> PAP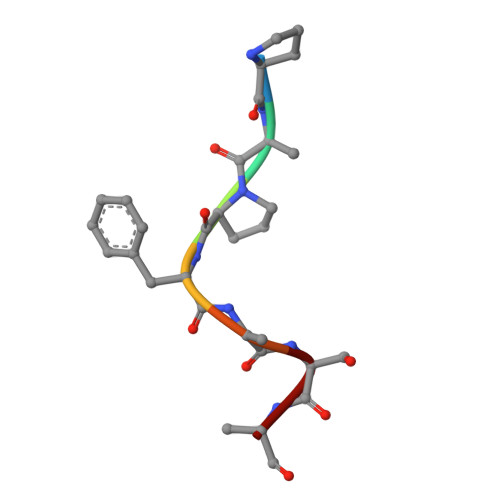FASA>GLVPRGSHMKVLVAEDQSMLRDAMCQLLTLQPDVESVLQAKNGQEAIQLLEKESVDIAILDVEMPVKTGLEVLEWIRSEKLETKVVVVTTFKRAGYFERAVKAGVDAYVLKERSIADLMQTLHTVLEGRKEYSPELMEMVMTRPNPLTEQEIAVLKGIARGLSNQEIAD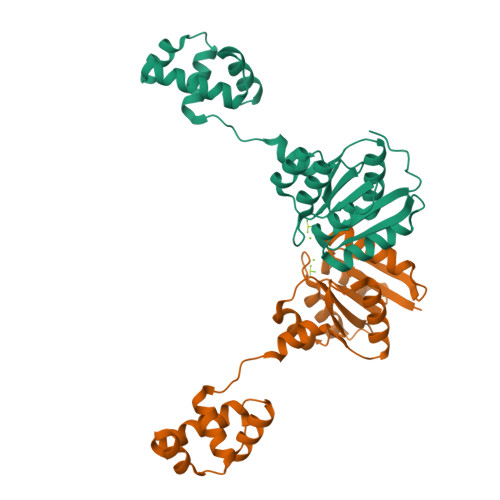QLYLSNGTIRNYVTNILSKLDAGNRTEAANIAKESGWL[2x]> M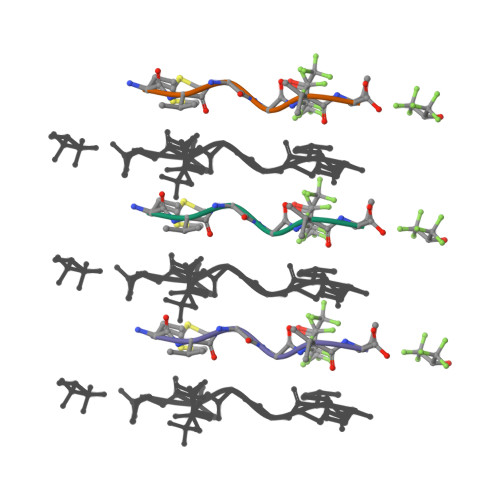VGGVV> GSGEAEERI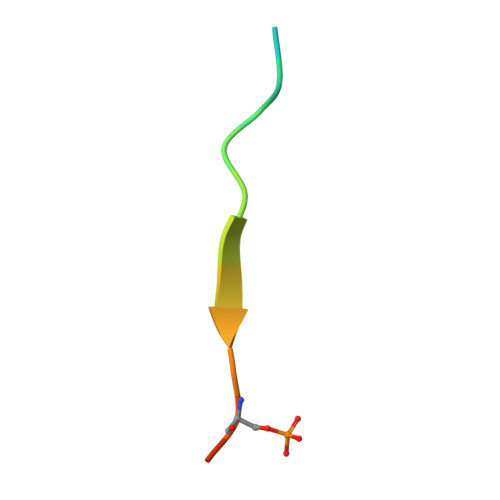IVLSDSDY1-PHENYLETHANONE | C8 H8 O | 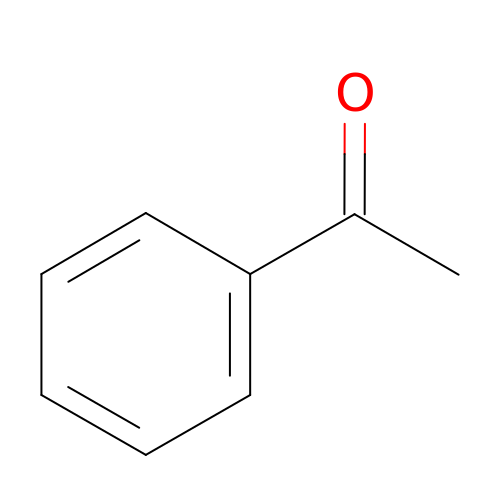KWOLFJPFCHCOCG-UHFFFAOYSA-N> GSMSTINFANREINFKIVYYGPGLSGKTTNLKWIYSKVPEGRKGE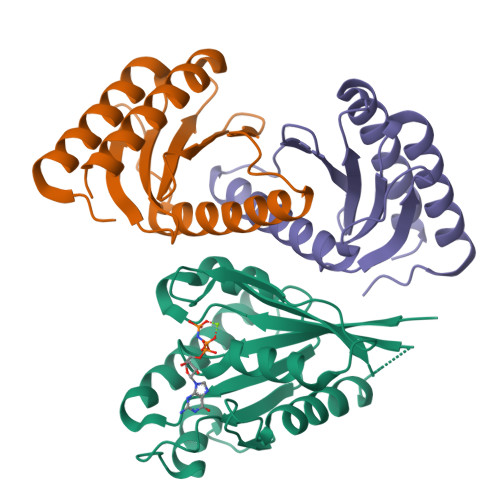MVSLATEDERTLFFDFLPLDIGEVKGFKTRFHLYTVPGQVFYNASRKLILRGVDGIVFVADSAPNRLRANAESMRNMRENLAEYGLTLDDVPIVIQVNKRDLPDALPVEMVRAVVDPEGKFPVLEAVATEGKGVFETLKEVSRLVLARVAGGS;>[2x]GSLVLYGAPYAAAVEVLEETLRETGARYALLIDRKGFVLAHKEALWAPKPPPLDTLATLVASNAAATQALAKLLGEARFQEEVHQGERMGLYVDEAGEHALLVLVFDETAPLGKVKLHGKAAAAALAAIAEEALAN>SAAEASKKPRQKRTATKAYNVTQAFGRRGPEQTQGNFGDQELIRQGTDYKHWPQIAQFAPSASAFFGMSRIGMEVTPS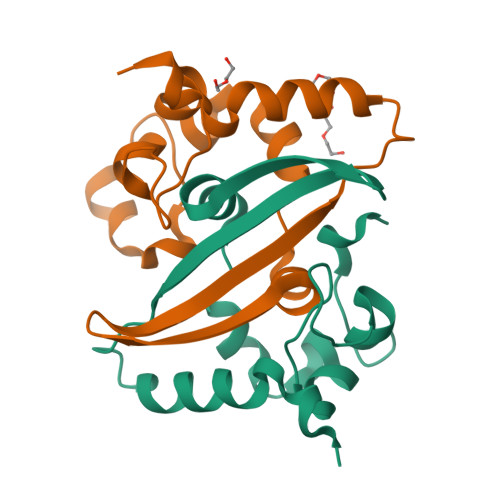GTWLTYTGAIKLDDKDPNFKDQVILLNKHIDAYKTFP[2x]>[2x]SGISLDNSYKMDYPEMGLCIIINNKNFHKSTGMTSRSGTDVDAANLRETFRNLK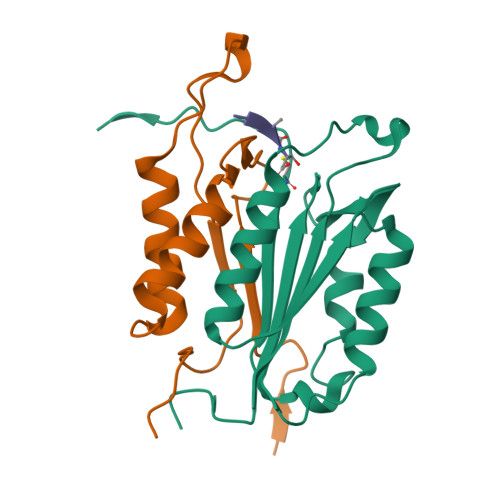YEVRNKNDLTREEIVELMRDVSKEDHSKRSSFVCVLLSHGEEGIIFGTNGPVDLKKITNFFRGDRCRSLTGKPKLFIIQACRGTEFDCGIETD;>SGVDDDMACHKIPVEADFLYAYSTAPGYYSWRNSKDGSWFIQSLCAMLKQYADKLEFMHILTRVNRKVATEFESFSFDATFHAKKQIPCIVSMLTKELYFYHHHHHHH[2x]>[2x]XGEIA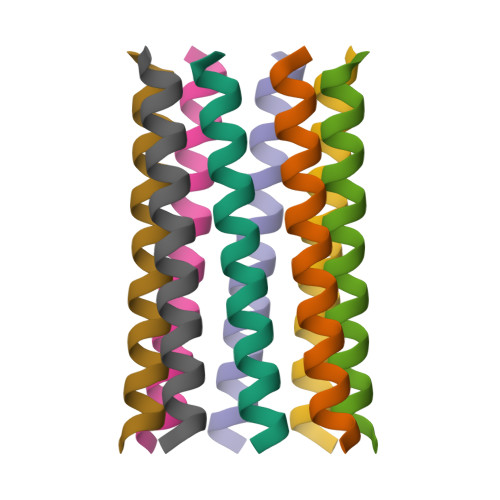QAYKEIAKALKEIAWALKEIAQALKGX> GMELPSFIFQAQENLVERPWGGEWIALLKGFRQSGIGESWEFSAHTSRPSTVLVKGQQLSMIELFSKHRDELLGRAAEKFSKFPILVRLIDAASPTQVHVHPSDKAAESLGEAEGGVESAWLVFNKGKAYAGFKEDVKIEELEEKLKEEDFDFKTLLNTFETTPYDTFVIRPGIPHAGEGLRVLEVSSNSTLAYFFNENDW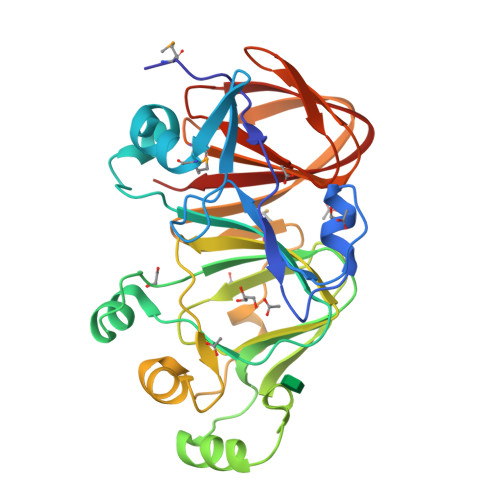EKVKKVLNTKKVEEFEVKGKKGMAETENFGLEVVDVTGTAEIKTGGVMNILYAAEGYFILRGKETADLHRGYSCLVPASTDSFTVESERGKIVRIYLKV>[2x]MRTILAGNGAFVLSDERGDMPSHYDGFYFLDTRFVRKARLEVSPEPDFIGASSTFTRAVSHFSLGERGILVRLRTLDGVYEEKLSFYNTSEESLGVKVRYSYEAPIEDIFQVRGFMGLKSGKAIAPAGGTHVKESPSGRRSLSIETNMEREGSLLRAELEIPPLGKAVLYVRFIPKIEGSISEILGEKRKTIKNVAFTGSPAIDGIFERAVENINALTLFTRFGPVPLAGIPYFACPFGRDAIIASLFLLPYYPEYAAGTLRLFGRLQGKRTNPKNEEEPGKIPHEFRLGELAQSGKVPFAPYYGTVDATPLYVALAGEYLRWTGDRKLIEELRPNLTAAVEWILKKLDDGYITYVPGILG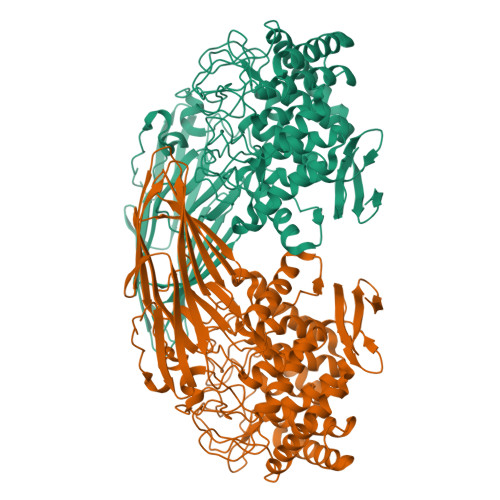NKGWKDSRDGIIDEEGKIPKPPIALVEVQGYTYWALKLAGELSLTDLDEKTLLAEAEKLKKRFNRDFWLGSYYALALDGEGRPLRVVSSNMGHLLLTGIAEHEEELAERLFRPDMFSRYGIRTLSAKEKAYNPFSYHRGSVWPHDNALIALGLARIGRTDMAKALMDAVFDAAKLLPERELPELYSGLNELVPVPRANSPQAWSSASVFAFVTASLGMEAGDELTVRPAEGTSIVLRGVSFGGRRYVVVVNGGVSVEPL The heterotrimeric RNA-dependent RNA polymerase (RdRp) of influenza virus is composed of subunits PA, PB1 and PB2. It is responsible for replication and transcription of the segmented, single-stranded viral RNA genome (vRNA) in the nucleus of infected cells. Transcription of viral mRNAs occurs through a unique “cap-snatching” mechanism. We initially screened metal-chelating compounds by CEN enzymatic assays, followed by a cellular phenotypic screen and then optimized the chemical structure to improve the pharmacokinetics and safety. This culminated in the generation of the compounds BXA and BXM that target the CEN in the PA proteins of influenza A and B viruses.

All four PA-BXA co-crystal structures exhibit clear and unambiguous electron density for the compound, which is bound in essentially the identical fashion in each structure. BXA has a butterfly like form, with one wing comprising a metal chelating polar oxazino-pyridotriazin-dione head-group and the other wing, a lipophilic, difluoro-dihydro-dibenzothiepine tail-group that makes van der Waals contacts with certain residues of the active site pocket. As expected, the head-group binds to the two divalent cations in the endonuclease active center, each metal ion having octahedral co-ordination through interactions with the protein, to the compound or water molecules, as previously described. In FluB wild-type, very similar interactions are made but with slightly different residues Thr20, Phe24, Met34, Asn37 and Ile38. The reduced size of Phe24 compared with Tyr24 allows Arg85 to change conformation and contact the compound in FluB but not FluA. Conserved Ile38 intimately packs into the V of the tail-group in identical fashion in both FluA and FluB, making van der Waals contacts via its CG1 and CD1 atoms. For the wild-type FluB endonuclease, the I38 side-chain conformation does not change upon ligand binding. In the absence of BXA, the Tm of all four endonuclease constructs is 46–50 °C. BXA binding to the endonuclease increases very significantly its thermal stability, with the Tm for the wild-type FluA or FluB endonuclease shifting to 78 or 77 °C, respectively, corresponding to ΔTm of +32 and +29 °C, respectively.

>GAMGSGMAMDTFITRNFQTTIIQKAKNTMAEFSEDPELQPAMLFNICVHLEVCYVISDMNFLDEEGKSYTALEGQGKEQNLRPQYEVIEGMPRTIAWMVQRSLAQEHGIETPKYLADLFDYKTKRFIEVGITKGLADDYFWKKKEKLGNSMELMIFSYNQDYSLSNESSLDEEGKGRVLSRLTELQAELSLKNLWQVLIGEEDVE[2x]>[2x]MGHHHHHHSIVKTMIVDDSAFMRNILKRILSTTNKYVVIGEAANGADAIKMAEELQPDLISMDIVMPETDGITATKAIKEKTPEIKIVMCTSVDQEQKMIDAVNAGADGYIVKPFQAPKILEQFNKLFPVLFQGPSAGLVPR;>GSGGIEGGSMGTIKSLLPKSEDDLDSEMAVESWSGDKLKNEVEQLAPEEQEILTAIYTGITSLELPGMMGMDIDEVEKVLEKLIDQGFLDLVRIRKETDLTEKGRAVTNFIITNF[2x]

In archaea, the adaptor protein CheF resides at the cytoplasmic face of the archaeal C-ring formed by the proteins ArlCDE and interacts with phosphorylated CheY. In archaea, CheY-P binds to CheF, an adaptor protein uniquely present in archaeal species, however the precise mechanism of this interaction is unclear to date. Binding of CheY-P to CheF induces a rotational switch of the archaellum. CheF forms a twisted homodimer offering two CheY-P binding sites within an elongated C-terminal tail domain.

We therefore constructed a fusion protein consisting of M. maripaludis CheY and the C-terminal 103 residues of CheF separated by a 20 amino acid linker including a thrombin cleavage site. We crystallized the CheY:CheFCTD in the presence of 2 mM BeF2 and 20 mM NaF (for more details, see Materials and methods section) and could solve the structure of this activated CheY:CheFCTD to a resolution of 2.3 Å, which allowed us to model both the full CheY-P and 70 amino acids of the CheFCTD into the electron density. A CheFCTD dimer bound to two CheY-P molecules was observed in the asymmetric unit. The interaction interface between CheY-P and CheFCTD involved the three helical bundle at CheFCTD with one molecule contributing α5 and α6 and the other one α8, covering a total of 778 Å2 buried surface area. At CheY-P, the interface mainly involves the regions directly adjacent to the BeF2 binding site, namely α1 and the β3-α4-loop as well as the β4-α5-loop. Comparing CheY-P to its non-activated form revealed that structural rearrangements upon activation mainly occur in the two mentioned loop regions and thus directly adjacent to the interaction interface with CheF. At CheF, conformational changes are mostly limited to helix α8 being kinked towards CheY-P upon binding. A closer inspection of the CheY-CheFCTD interaction showed that the interaction is mostly mediated by hydrophobic residues and some polar backbone contacts “clamping” the interface on one side. Interestingly, the terminal carboxyl-moiety of MmCheF F348 reaches into the phosphorylation site contacting one of the waters coordinating the Mg2+ and MmCheY K107. We show that two CheY-P molecules bind to the dimeric CTD of CheF involving an interface near the phosphorylation site of CheY thus allowing a direct sensing of the phosphorylation state of CheY by CheF.>MALSTATKAATDALAANRAPTSVNAQEVHRWLQSFNWDFKNNRTKYATKYKMANETKEQFKLIAKEYARMEAVKDERQFGSLQDALTRLNAGVRVHPKWNETMKVVSNFLEVGEYNAIAATGMLWDSAQAAEQKNGYLAQVLDEIRHTHQCAYVNYYFAKNGQDPAGHNDARRTRTIGPLWKGMKRVFSDGFISGDAVECSLNLQLVGEACFTNPLIVAVTEWAAANGDEITPTVFLSIETDELRHMANGYQTVVSIANDPASAKYLNTDLNNAFWTQQKYFTPVLGMLFEYGSKFKVEPWVKTWDRWVYEDWGGIWIGRLGKYGVESPRSLKDAKQDAYWAHHDLYLLAYALWPTGFFRLALPDQEEMEWFEANYPGWYDHYGKIYEEWRARGCEDPSSGFIPLMWFIENNHPIYIDRVSQVPFCPSLAKGASTLRVHEYNGEMHTFSDQWGERMWLAEPERYECQNIFEQYEGRELSEVIAELHGLRSDGKTLIAQPHVRGDKLWTLDDIKRLNCVFKNPVKAFN[2x];>[2x]SMLGERRRGLTDPEMAEVILKALPEAPLDGNNKMGYFVTPRWKRLTEYEALTVYAQPNADWIAGGLDWGDWTQKFHGGRPSWGNETTELRTVDWFKHRDPLRRWHAPYVKDKAEEWRYTDRFLQGYSADGQIRAMNPTWRDEFINRYWGAFLFNEYG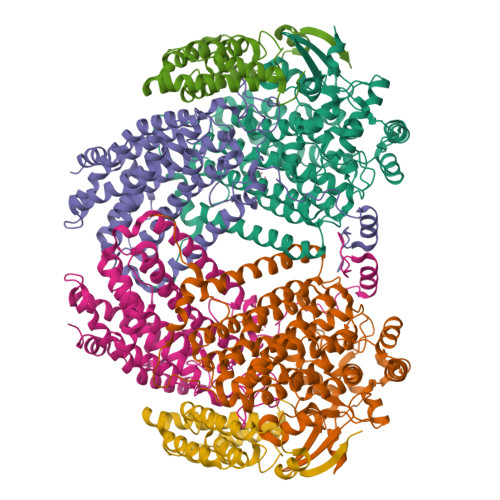LFNAHSQGAREALSDVTRVSLAFWGFDKIDIAQMIQLERGFLAKIVPGFDESTAVPKAEWTNGEVYKSARLAVEGLWQEVFDWNESAFSVHAVYDALFGQFVRREFFQRLAPRFGDNLTPFFINQAQTYFQIAKQGVQDLYYNCLGDDPEFSDYNRTVMRNWTGKWLEPTIAALRDFMGLFAKLPAGTTDKEEITASLYRVVDDWIEDYASRIDFKADRDQIVKAVLAGLK;>AKLGIHSNDTRDAWVNKIAQLNTLEKAAEMLKQFRMDHTTPFRNSYELDNDYLWIEAKLEEKVAVLKARAFNEVDFRHKTAFGEDAKSVLDGTVAKMNAAKDKWEAEKIHIGFRQAYKPPIMPVNYFLDGERQLGTRLMELRNLNYYDTPLEELRKQRGVRVVHLQSPH[2x]> PHMPPLPPGWEEKVDNLGRTYYVNHN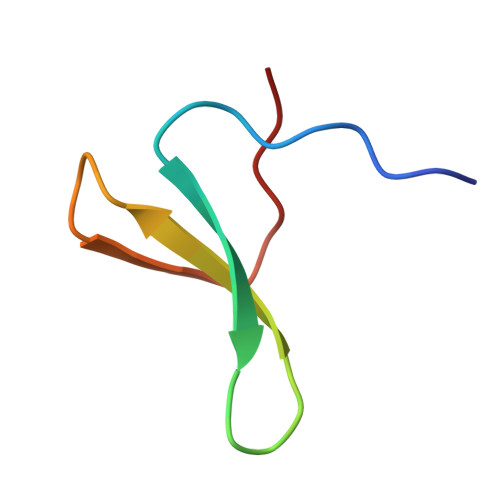NRTTQWHRPSL>[16x]AAFVKENHRQLQ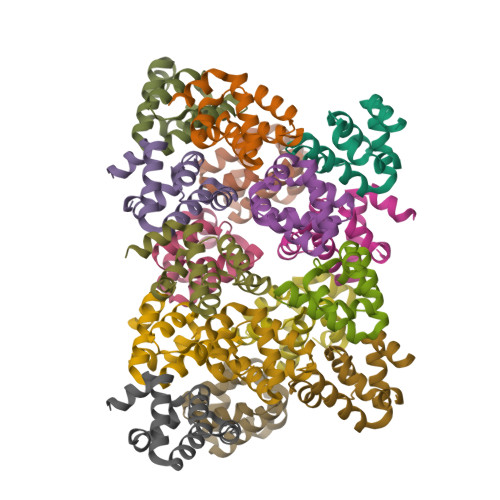ARMGDLKGVLDDLQDNEVLTENEKELVEQEKTRQSKNEALLSMVEKKGDLALDVLFRSISERDPYLVSYLRQQNL>[4x]MSAKAISEQTGKELLYKFICTTSAIQNRFKYARVTPDTDWARLLQDHPWLLSQNLVVKPDQLIKRRGKLGLVGVNLTLDGVKSWLKPRLGQEATVGKATGFLKNFLIEPFVPHSQAEEFYVCIYATREGDYVLFHHEGGVDVGDVDAKAQKLLVGVDEKLNPEDIKKHLLVHAPEDKKEILASFISGLFNFYEDLYFTYLEINPLVVTKDGVYVLDLAAKVDATADYICKVKWGDIEFPPPFGREAYPEEAYIADLDAKSGASLKLTLLNPKGRIWTMVAGGGASVVYSDTICDLGGVNELANYGEYSGAPSEQQTYDYAKTILSLMTREKHPDGKILIIGGSIANFTNVAATFKGIVRAIRDYQGPLKEHEVTIFVRRGGPNYQEGLRVMGEVGKTTGIPIHVFGTETHMTAIVGMALGHRPIPNQPPTAAHTANFLLNASGSTSTPAPSRTASFSESRADEVAPAKKAKPAMPQDSVPSPRSLQGKSTTLFSRHTKAIVWGMQTRAVQGMLDFDYVCSRDEPSVAAMVYPFTGDHKQKFYWGHKEILIPVFKNMADAMRKHPEVDVLINFASLRSAYDSTMETMNYAQIRTIAIIAEGIPEALTRKLIKKADQKGVTIIGPATVGGIKPGCFKIGNTGGMLDNILASKLYRPGSVAYVSRSGGMSNELNNIISRTTDGVYEGVAIGGDRYPGSTFMDHVLRYQDTPGVKMIVVLGEIGGTE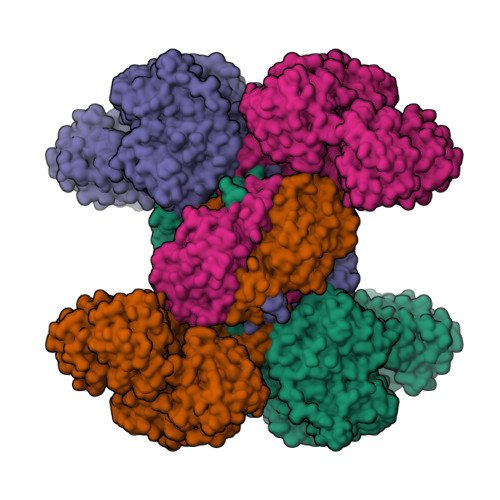EYKICRGIKEGRLTKPIVCWCIGTCATMFSSEVQFGHAGACANQASETAVAKNQALKEAGVFVPRSFDELGEIIQSVYEDLVANGVIVPAQEVPPPTVPMDYSWARELGLIRKPASFMTSICDERGQELIYAGMPITEVFKEEMGIGGVLGLLWFQKRLPKYSCQFIEMCLMVTADHGPAVSGAHNTIICARAGKDLVSSLTSGLLTIGDRFGGALDAAAKMFSKAFDSGIIPMEFVNKMKKEGKLIMGIGHRVKSINNPDMRVQILKDYVRQHFPATPLLDYALEVEKITTSKKPNLILNVDGLIGVAFVDMLRNCGSFTREEADEYIDIGALNGIFVLGRSMGFIGHYLDQKRLKQGLYRHPWDDISYVLPEHMS>TYTTRQIGAKNTLEYKVYIEKDGKPVSAFHDIPLYADKENNIFNMVVEIPRWTNAKLEITKEETLNPIIQDTKKGKLRFVRNCFPHHGYIHNFGAFPQTWEDPNVSHPETKAVGDNDPIDVLEIGETIAYTGQVKQVKALGIMALLDEGETDWKVIAIDINDPLAP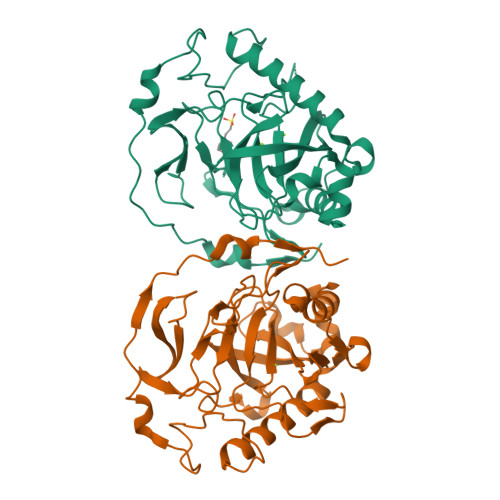KLNDIEDVEKYFPGLLRATNEWFRIYKIPDGKPENQFAFSGEAKNKKYALDIIKETHDSWKQLIAGKSSDSKGIDLTNVTLPDTPTYSKAASDAIPPASLKADAPIDKSIDKWFFISGSV[2x]> MFFQIEKVVLWSKEAKHKPRVIEFALNKVNLITGSSKSGKSSLIPIIDYCLGSSKCSIPVNTIRDTTAWYGVQIKTKHSRLLIARRDPSNQLSTSNAFFVEAENIEIPQNIEKHNVNIDTVKNRLNEISGVSNISFDFYDTGRIDKKRTSTRDLSAFNYQPQNIIANPNALFYKTDSFEHKSKLVTILPYVLGALSNTDIENQHRIKNLEEEYRKVERRLLKLKRQNEDWLSSAQAYVIKAMELGLVNSDKDIYQLKPERLLNVLKNIATKEIDYSTSAANIKYASEQEAEITKRSRDISNNLAKVKSRLQNINSMNRLANTHSDASRLKRERLSLSKWLLTQNDINSSLFSEPNEIRSLVLEPLARAFSNLEAELEVPIHVQGALSREKIYLEGELTRLASEMKDVNTQLKILRGNKRKLGYDAFSVGKFVGEVEKALSLMGESESESELSKEYKRLKKELSVLRLKIDPREFERKTKLQLAKVNKLASDWLPHLDTENPNAPISLHEKELTITVNSSGREDYLWEIGSGANWLSYHVAITLALHQHFSSLEASPVPNYIIYDQPSQVYFPSKLRHQATPEEDELALLEQDEDIVQVKKIFEAFNGAIEKTKDNLQIIVLDHAPSTLVKSIPKGHLVEEWRNGI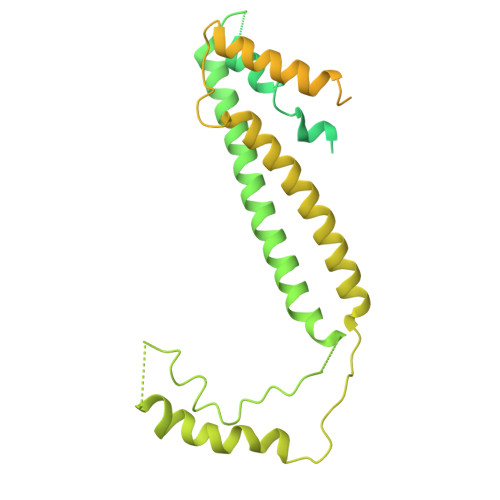KLIPLDWL> DSIVVAYYFCGEPIP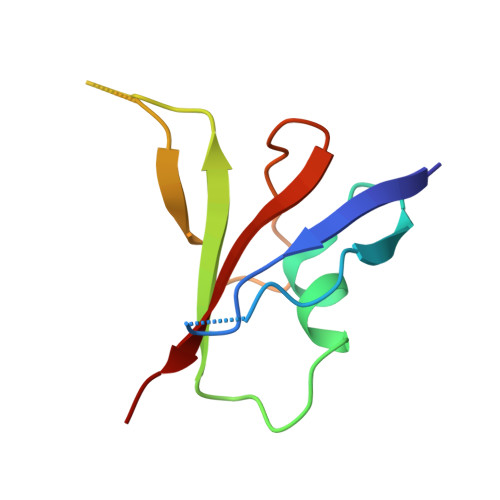DRTLVRGRAVTLGQFKELLTKKGSYRYYFKKVSDEFDCGVVFEEVREDEAVLPVFEEKIIGKVEKVD(2~{S})-2-oxidanyl-3-oxidanylidene-butanedioic 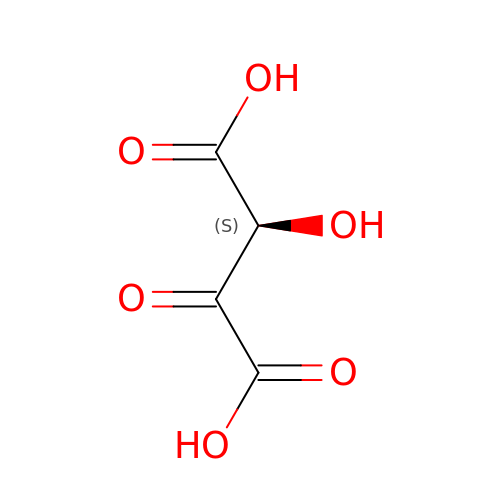acid | C4 H4 O6 | RMHHUKGVZFVHED-SFOWXEAESA-N> MASISSLGVGSNLPLDQLLTDLTKNEKGRLTPITKQQSANSAKLTAYGTLKSALEKFQTANTALNKADLFKSTVASSTTEDLKVSTTAGAAAGTYKINVTQLAAAQSLATKTTFATTKEQLGDTSVTSRTIKIEQPGRKEPLEIKLDKGDTSMEAIRDAINDADSGIAASIVKVKENEFQLVLTANSGTDNTMKITVEGDTKLNDLLAYDSTTNTGNMQELVKAENAKLNVNGIDIERQSNTVTDAPQGITLTLTKKVTDATVTVTKDDTKAKEAIKSWVDAYNSLVDTFSSLTKYTAV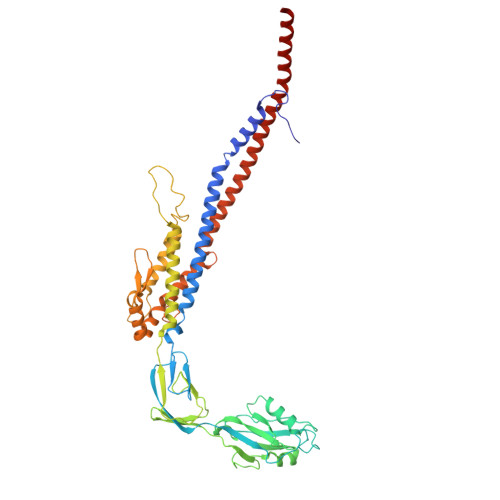EPGEEASDKNGALLGDSVVRTIQTGIRAQFANSGSNSAFKTMAEIGITQDGTSGKLKIDDDKLTKVLKDNTAAARELLVGDGKETGITTKIATEVKSYLADDGIIDNAQDNVNATLKSLTKQYLSVSNSIDETVARYKAQFTQLDTMMSKLNNTSSYLTQQFTAMNKS>[2x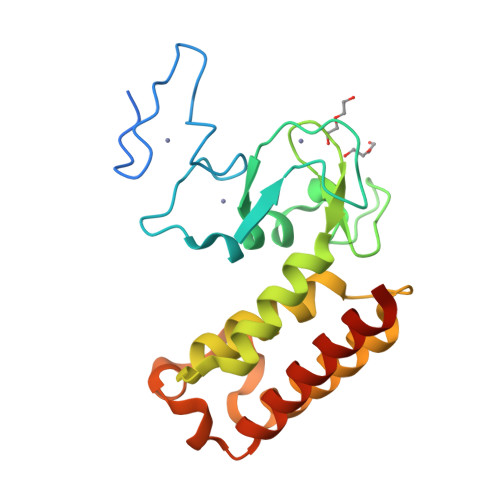]GPDSMPLKRKEEQVDTLICQNLACRATLSLEDGYCKRCSCCICHCYDENKDPSLWLVCNSDPPYLSNSCGMSCHLKCALKHETAGILKNGCYPKLDGSFYCVFCGKVNWLIGSWRKQLLIAKDARRVDVLCDRLSLSHKMLKGTEHYKDMQNIVNTAVKKLKKEVGPLDKVSAVMARGIVNRLNCGTEVQKLCVSAVEAADSMLSSSTD> GHMQETQAVEAGEKTVEQFVQALNKGDYNKAAEMTSKKAANKSALSEKEILDKYQNIYGAADVKGLQISNLKVDKKDDSTYSFSYKAKMNTSLGELKDLSYKGTLDRNDGQTTINWQPNLVFPEMEGNDKVSLTTQEAARGNIIDRNGEPLATTGKLKQLGVVPSKLGDGGEKTANIKAIASSFDLTEDAINQAISQSWVQPDYFVPLKIIDGATPELP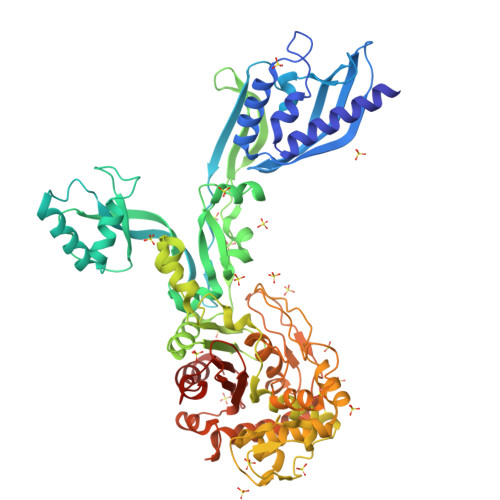AGATIQEVDGRYYPLGEAAAQLIGYVGDITAEDIDKNPELSSNGKIGRSGLEMAFDKDLRGTTGGKLSITDADGVEKKVLIEHEVQNGKDIKLTIDAKAQKTAFDSLGGKAGSTVATTPKTGDLLALASSPSYDPNKMTNGISQEDYKAYEENPEQPFISRFATGYAPGSTFKMITAAIGLDNGTIDPNEVLTINGLKWQKDSSWGSAQVTRVSDVSQVDLKTALIYSDNIYTAQETLKMGEKKFRTGLDKFIFGEDLDLPISMNPAQISNEDSFNSDILLADTGYGQGELLINPIQQAAMYSVFANNGTLVYPKLIADKETKDKKNVIGETAVQTIVPDLREVVQDVNGTAHSLSALGIPLAAKTGTAEIKEKQDVKGKENSFLFAFNPDNQGYMMVSMLENKEDDDSATKRASELLQYLNQNYQ>MEKVPGEMEIERRERSEELSEAERKAVQAMWARLYANSEDVGVAILVRFFVNFPSAKQYFSQFKHMEDPLEMERSPQLRKQASRVMGALNTVVENLHDPDKVSSVLALVGKAHALKHKVEPVYFKILSGVILEVVAEEFASDFPPETQRAWAKLRGLIYSHVTAAYKEVG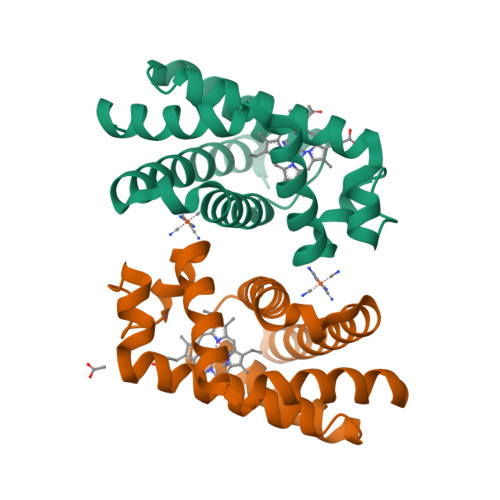WVQQVPNATTPPATLPSSGP[2x]> GPAVPRMVIEDFALNLELFRLINNARHPLLDVFFTHFAYLGSGYVLFPLLIFLFIFRKEKVKPLILAIMLETVLVISLKTFFNQPRPAILLEDVNLLFPLHWRSFPSGDTAMAFTIATVLSHGEKLHIKAILFLYAFLIGYERIYAGVHFPLDVFVGALIGIIC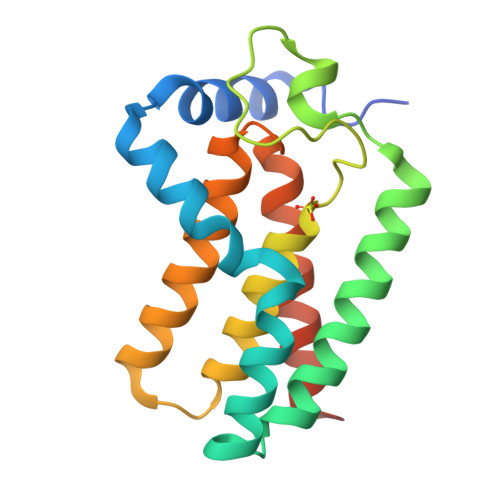GIISLKYSKGGVYERN Computational design of KE07 involved construction of a theozyme to catalyze the chemical reaction, which was then grafted into the scaffold of imidazole glycerol phosphate synthase (HisF) from Thermotoga maritima. Catalytically essential residues from the initial design include a base (Glu101) that facilitates C−H bond cleavage, an H-bond donor (Lys222) to stabilize the phenoxide intermediate, and a π-stacking residue (Trp50), which was designed to stabilize the transition state and favor substrate binding through interactions with the aromatic ring of the substrate. This initial KE07 design (Round 1; R1) catalyzes the cleavage of 5-nitrobenzisoxazole, with 103-fold rate acceleration over the noncatalyzed reaction and a turnover rate (kcat) of 0.018 s−1.

Thus, the mechanism by which the remote mutations that appear in R5 and R6 increase activity is qualitatively different. This is mirrored in their location within the protein; in contrast to the initial mutations that affect the active site directly, the mutations in R5 (Val12Met) and R6 (Lys146Thr) are remote from the active site. The Val12Met and Phe77Ile mutations, also in the second shell, cause changes to internal cavities that cause a slight rotation in the backbone at Trp50 that also favors the alternative configuration. To the solution sampling of these states, we used HREX-MD simulations, which are among the most comprehensive computational methods to investigate conformational sampling. These results were consistent with the crystallography and kinetic analysis: whereas in R1 (original design), configuration A was the dominant substate that was sampled, by R5 we observe increased sampling of configurations B and C. By R7 and R7-2, configuration C (which was the only state we saw associated with product in the crystal structures) becomes the dominant substate sampled, with configurations A and B sampled only rarely. These simulations also reveal that the mobility of Glu101 was reduced as a result of the hydrogen bond formed to the indole nitrogen of Trp50 in R5; this could account for the improved pre-exponential factor from R5 onwards.

> MALAKRIDAALIMKDGRVVKGSNFENLRDSGDPVELGKFYSEIGIDELSFWDITASVEKRKTMLELVEKVAEQIDIPFTVGGGIHDFETASELILRGADKVEINTAAVENPSLITQIAQTFGSQAVVVYIAAKRVDGEFMVFTYSGKKNTGILLRDWVVEVEKRGAGEIVLGSIDRLGTKSGYDTEMIRFVRPLTTLPIIAHRGAGKMEHFLEAFLAGADAAKADSVFHFREIDVRELKEYLKKHGVNVRLEGLGSLEHHHHHH>[4x]GCAGCAGC

We have analyzed crystal structures of RNA containing CAG repeats in complex with synthetic cyclic mismatch-binding ligands (CMBLs). In total, three X-ray structures consisting of (GCAGCAGC)2-CMBL3a, one structure of (GCAGCAGC)2-CMBL3b and one (GCAGCAGC)2-CMBL4 complex have been analyzed. The models show well-defined interactions between the molecules in which the CMBLs mimic nucleobases as they form pseudo-canonical base pairs with adenosine residues and engage in extensive stacking interactions with neighboring nucleotides. The binding of ligands is associated with major structural changes of the CAG repeats, which is consistent with results of biochemical studies.

The longer linker contains two N-acyl-amino groups and additional constituents: in CMBL3a it is a E-alkene, in CMBL3b it is an Z-alkene, and in CMBL4 it is an aminoalkyl moiety. Alternatively, in the CAG-CMBL3a(I), the flipped out 4G and 5C residues form an i-motif like structure consisting of C–C+ and G–G pairs. The two nucleobases engage in H-bonding via their Watson–Crick edges are oriented in trans relative to the N-glycosidic bonds, resulting in the parallel orientation of the RNA chains. In the presence of CMBL3a, the duplex is the most stable, having a melting temperature TM nearly 20°C higher. The X-ray structures show that all three ligands interact with the RNA in very similar manners, but the conformation of the bound CMBL3a is the least distorted from the idealized geometry. The asymmetric trans conformation of the long linker makes the ligand better adjusted to the binding site than the symmetric CMBL3b and CMBL4. This is consistent with the thermal melting observations that CMBL3a forms more stable complexes with the RNA than CMBL3b or CMBL4. Circular dichroism (CD) spectra of (CAG)9 showed a clear conformational change upon CMBL3a binding.> MPPGVDCPMEFWTKEESQSVVVDFLLPTGVYLNFPVSRNANLSTIKQVLWHRAQYEPLFHMLSDPEAYVFTCVNQTAEQQELEDEQRRLCDIQPFLPVLRLVAREGDRVKKLINSQISLLIGKGLHEFDSLRDPEVNDFRTKMRQFCEEAAAHRQQLGWVEWLQYSFPLQLEPSARGWRAGLLRVSNRALLVNVKFEGSEESFTFQVSTKDMPLALMACALRKKATVFRQPLVEQPEEYALQVNGRHEYLYGNYPLCHFQYICSCLHSGLTPHLTMVHSSSILAMRDEQSNPAPQVQKPRAKPPPIPAKKPSSVSLWSLEQPFSIELIEGRKVNADERMKLVVQAGLFHGNEMLCKTVSSSEVNVCSEPVWKQRLEFDISVCDLPRMARLCFALYAVVEKAKKARSTKKKSKKADCPIAWANLMLFDYKDQLKTGERCLYMWPSVPDEKGELLNPAGTVRGNPNTESAAALVIYLPEVAPHPVYFPALEKILELGRHGERGRITEEEQLQLREILERRGSGELYEHEKDLVWKMRHEVQEHFPEALARLLLVTKWNKHEDVAQMLYLL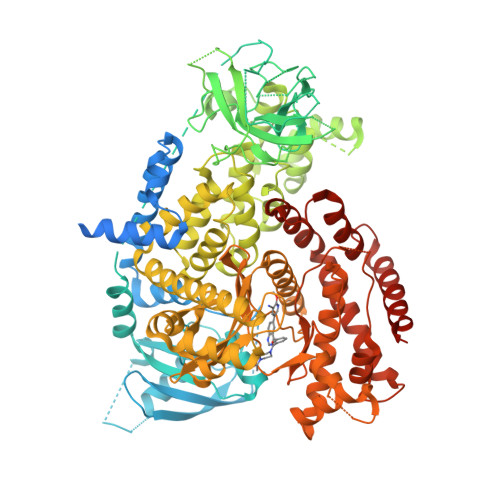CSWPELPVLSALELLDFSFPDCYVGSFAIKSLRKLTDDELFQYLLQLVQVLKYESYLDCELTKFLLGRALANRKIGHFLFWHLRSEMHVPSVALRFGLIMEAYCRGSTHHMKVLMKQGEALSKLKALNDFVKVSSQKTTKPQTKEMMHMCMRQETYMEALSHLQSPLDPSTLLEEVCVEQCTFMDSKMKPLWIMYSSEEAGSAGNVGIIFKNGDDLRQDMLTLQMIQLMDVLWKQEGLDLRMTPYGCLPTGDRTGLIEVVLHSDTIANIQLNKSNMAATAAFNKDALLNWLKSKNPGEALDRAIEEFTLSCAGYCVATYVLGIGDRHSDNIMIRESGQLFHIDFGHFLGNFKTKFGINRERVPFILTYDFVHVIQQGKTNNSEKFERFRGYCERAYTILRRHGLLFLHLFALMRAAGLPELSCSKDIQYLKDSLALGKTEEEALKHFRVKFNEALRESWKTKVNWLAHNVSKDNRQ> TETTSFSITKFGPD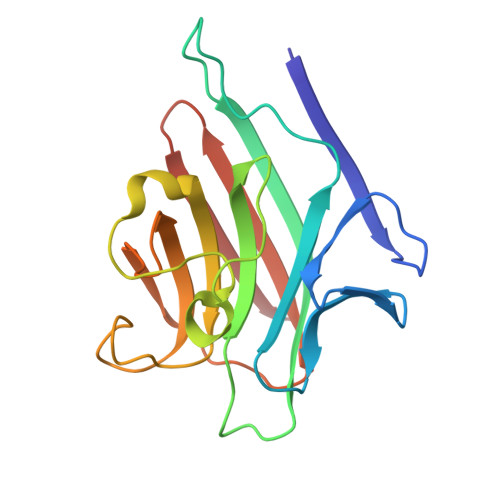QPNLIFQGDGYTTKERLTLTKAVRNTVGRALYSSPIHIWDSKTGNVANFVTSFTFVIDAPNSYNVADGFTFFIAPVDTKPQTGGGYLGVFNSKDYDKTSQTVAVEFDTFYNTAWDPSNGDRHIGIDVNSIKSINTKSWKLQNGKEANVVIAFNGATNVLTVSLTYPN> TIQNDIPDLYSVFKDYFPIGVAVDPSRLNDADPHAQLTAKHFNMLVAENAMKPESLQPTEGNFTFDNADKIVDYAIAHNMKMRGHTLLWHNQVPDWFFQDPSDPSKPASRDLLLQRLRTHITTVLDHFKTKYGSQNPIIGWDVVNEVLDDNGNLRNSKWLQIIGPDYIEKAFEYAHEADPSMKLFINDYNIENNGVKTQAMYDLVKKLKNEGVPINGIGMQMHISINSNIDNIKASIEKLASLGVEIQVTALDM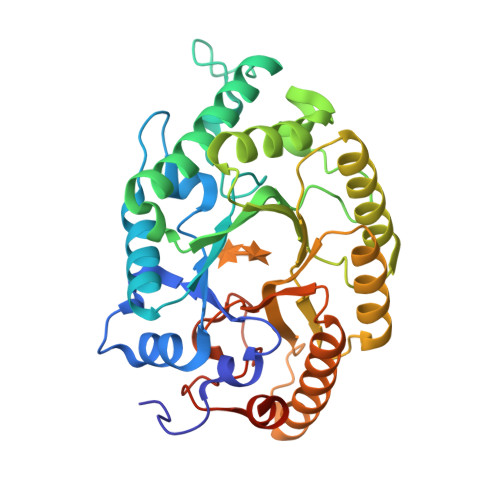NMNGDVSNDALLKQARLYKQLFDLFKAEKQYITAVVFWGVSDDVSWLSKPNAPLLFDSKLQAKPAYWAIVDLGKAIPDIQSA>HHHMSEATLLSYTKKLLASPPQLSSTDLHDALLVILSLLQKCDTNSDESLSIYTKVSSFLTALRVTKLDHKAEYIAEAAKAVLRHSDLVDLPLPKKDELHPEDGPVILDIVGTGGDGQNTFNVSTSAAIVASGIQGLKICKHGGKASTSNSGAGDLIGTLGCDMFKVNSSTVPKLWPDNTFMFLLAPFFHHGMGHVSKIRKFLGIPTVFNVLGPLLHPVSHVNKRILGVYSKELAPEYAKAAALVYPGSETFIVWGHVGLDEVSPIGKTTVWHIDPTSSELKLKTFQLEPSMFGLEEHELSKCASYGPKEN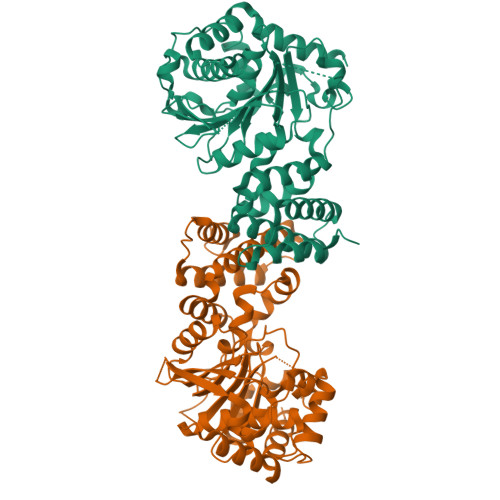ARILKEEVLSGKYHLGDNNPIYDYILMNTAVLYCLSQGHQNWKEGIIKAEESIHSGNALRSLEHFIDSVSSL[2x]> AASFI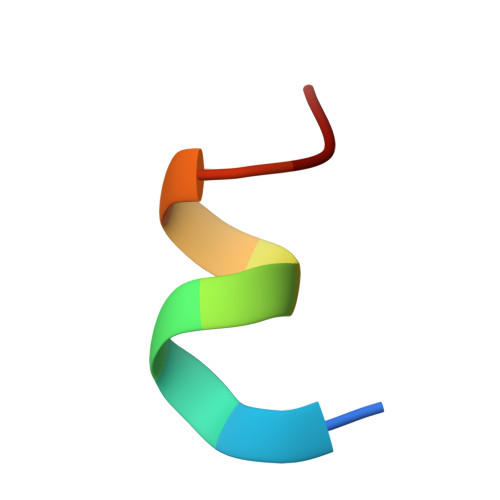DAKKMP>EYAPSPLDWSREQADTYMKSGGTEGTQLQGKPVILLTTVGAKTGKLRKTPLMRVEHDGQYAIVASLGGAPKNPVWYHNVVKNPRVELQDGTVTGDYDAREVFGDEKAIWWQRAVAVWPDYASYQTKTD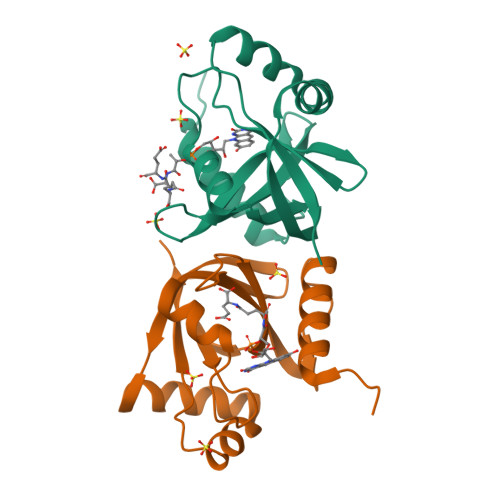RQIPVFVLTPVR[2x]>[2x]GSHMAGTALKRLMAEYKQLTLNPPE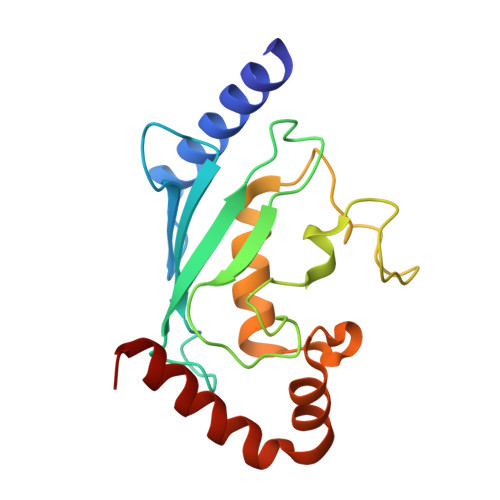GIVAGPMNEENFFEWEALIMGPEDTCFEFGVFPAILSFPLDYPLSPPKMRFTCEMFHPNIYPDGRVCISILHAPGDDPMGYESSAERWSPVQSVEKILLSVVSMLAEPNDESGANVDASKMWRDDREQFYKIAKQIVQKSLGL;> SADERQRMLVQRKDELLQQARKRFLNKS>MAVSDSQNSQTCLDPDASRSVLGIILGGGAGTRLYPLTKKRAKPAVPLGANYRLIDIPVSNCLNSNISKIYVLTQFNSASLNRHLSRAYASNMGGYKNEGFVEVLAAQQSPENPDWFQGTADAVRQYLWLFEEHTVLEYLILAGDHLYRMDYEKFIQAHRETDADITVAALPMDEKRATAFGLMKIDEEGRIIEFAEKPQGEQLQAMKVDTTILGLDDKRAKEMPFIASMGIYVISKDVMLNLLRDKFPGANDFGSEVIPGATSLGMRVQAYLYDGYWEDIGTIEAFYNANLGITKKPVPDFSFYDRSAPIYTQPRYLPPSKMLDADVTDSVIGEGCVIKNCKIHHSVVGLRSCISEGAIIEDSLL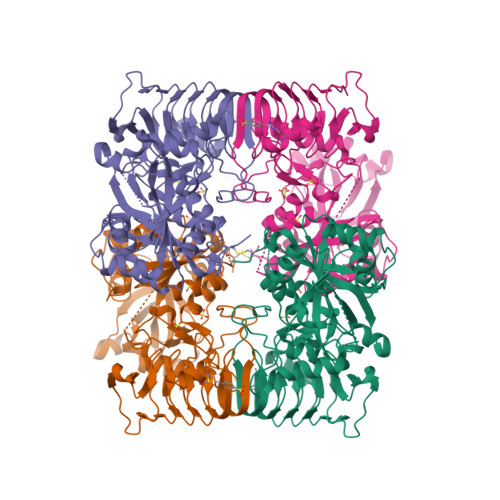MGADYYETDADRKLLAAKGSVPIGIGKNCHIKRAIIDKNARIGDNVKIINKDNVQEAARETDGYFIKSGIVTVIKDALIPSGIII[4x]> MEQKLISEEDLNEMEQKLISEEDLNEMEQKLISEEDLNEMEQKLISEEDLNEMEQKLISEEDLNEMESLGDLTMEQKLISEEDLNSGRPAAMAQVINTNVASLTAQRNLGVSGNMMQTSIQRLSSGLRINSAKDDAAGLAISQRMTAQIRGMNQAVRNANDGISLAQVAEGAMQETTNILQRMRELSVQAANSTNNSSDRSSIQSEISQLK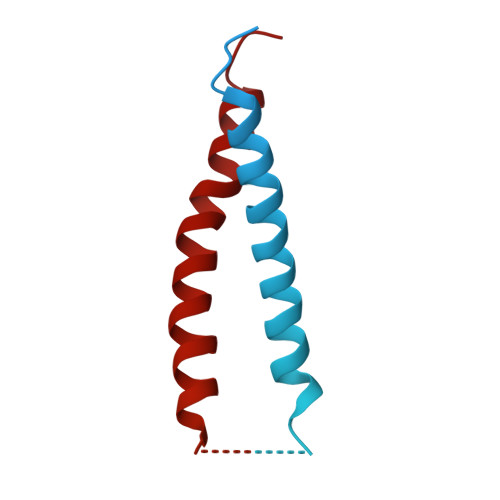SELERIAQNTEFNGQRILDGSFSGASFQVGANSNQTINFSIGSTKASSLGGIATATGTEVAGAAAADITIAIGGGAATSINSSANFTGALNGQDATSAYAKAAAINDAGIGGLSVTASTSGTQAVGAIGGTAGDTYNLTINGVAIYTNLNVATALTNSDLRDAINGVSNQTGVVASLNGGNMTLTAADGRNITVTESGTGFTAGTDGLTVTGGAFDGALRGTLSISAVDTIAIGGTVANIGLSANISKDTVGIDSLDVSTASGAQTAIKRIDAALNSVNSNRANMGALQNRFESTIANLQNVSDNLSAARSRIQDADYAAEMASLTKNQILQQAGTAMLAQANSLPQSVLSLLGR>RMSDGAAPKANGSEASGQDLVPAAVEQAVPIQPVAGAALAAPAAGQINQIDPWIFQNFVQCPLGEFSISPRNTPGEILFDLALGPGLNPYLAHLSAMYTGWVGNMEVQLVLAGNAFTAGKVVVALVPPYFPKGSLTTAQITCFPHVMCDVRTLEPIQLPLLDVRRVLWHATQDQEESMRLVCMLYTPLRTNSPGDESFVVSGRLLSKPAADFNFVYLTPPIERTIYRMVDLPVIQPRLCTHARWPAPVYGLLVDPSLPSNPQWQNGRVHVDGTLLGTTPISGSWVSCFAAEAAYEFQSGTGEVATFTLIEQDGSAYVPGDRAAPLGYPDFSGQLEIEIQTETTKTGDKLKVTTFEMILGPTTNADQAPYQGRVFASVTAAASLDLVDGRVRAVPRSIYGFQDTIPEYNDGLLVPLAPPIGPFLPGEVLLRFRTYMRQIDTADAAAEAIDCALPQEFVSWFASNAFTVQSEALLLRYRNTLTGQLLFECKLYNEGYIALSYSGSGPLTFPTDGIFEVVSWVPRLYQLASVGSLATGRMLKQ[3x]

The T=3 icosahedral calicivirus capsid is composed of 180 copies of VP1 with a molecular weight of ~58 kDa, which is divided into the N-terminus (N), the shell (S) and the C-terminal protruding (P) domain (1–5). The S domain forms a shell around the viral RNA genome, while the P domains form protrusions emanating from the shell comprising A/B and C/C dimers. The P domain is further subdivided into P1 and P2 subdomains, with the latter containing the binding sites for cellular receptors and neutralizing antibodies. At conditions found in the gut (i.e., low pH with high metal ion and bile salt concentrations), the P domain rotates and drops onto the shell with intra P domain changes that enhance receptor interactions while blocking antibody binding.

Once the sequence of the purified mutant virus had been verified to contain the V339I mutation, the structures of V339I apo, V339I + 2 mM CaCl2, and V339I + 10 mM GCDCA were determined from that same sample. The calculated resolutions for all three cryo-EM reconstructions were ~2.7Å. Panel A shows an overlay of V339I apo (blue and green) onto V339I+GCDCA (red and orange). The positions of the P domains are essentially identical and are in the activated state, resting on the shell surface. The overall RMSD of the alignment between these two structures is ~0.4Å, well within the margin of error at this resolution. The only apparent differences between the two structures are in the outermost loops that are more than likely due to inherent flexibility. The correlation coefficients are calculated during real space refinement in PHENIX and represent the agreement between the refined model and real space density. These outermost loops become more ordered with the addition of GCDCA or Ca2+ (the color shifts from reds/yellows to blues/greens), which is likely due to the stabilized positions of the G’H’/C’D’ loops (insets in Fig. 5A through C). The addition of activators (i.e., GCDCA or CaCl2+) decreased the mobility of this P2 domain as per the improved CC. Therefore, while the V339I mutation alone is sufficient to push the P domain nearly into the fully activated conformation, the addition of these activators finishes the activation process and stabilizes these key loops.>MRPPFTYATLIRWAILEAPEKQRTLNEIYHWFTRMFAFFRNHPA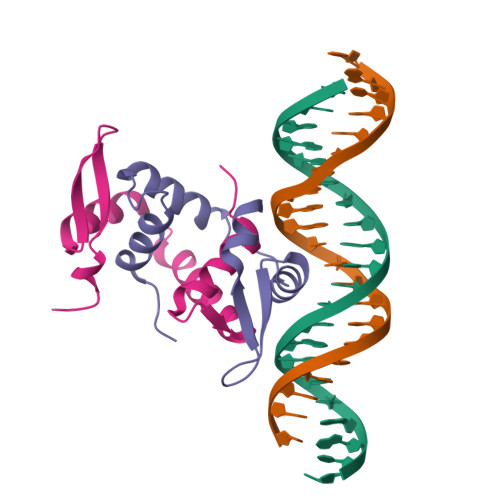TWKNAIRHNLSLHKCFVRVESEKGAVWTVDELEFRKKR[2x]>[6x]MKTHKTKNDLPSNAKSTVIGILNESLASVIDLALVTKQAHWNLKGPQFIAVHELLDTFRTQ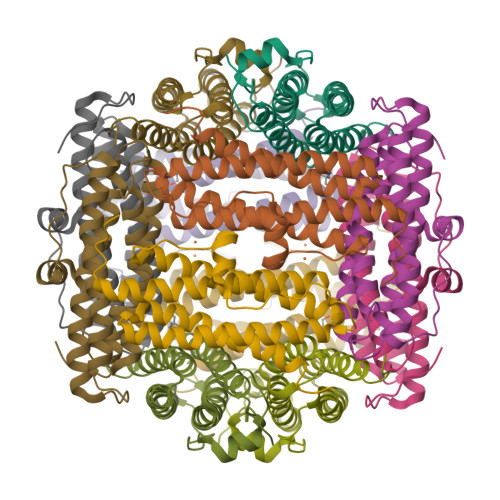LDNHGDTIAERVVQLGGTALGSLQAVSSTTKLKAYPTDIYKIHDHLDALIERYGEVANMIRKAIDDSDEAGDPTTADIFTAASRDLDKSLWFLEAHVQEKS> MPSQN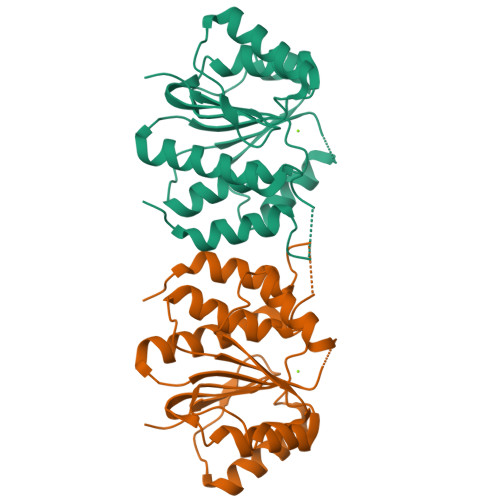ALYLDLLKKVLTNTIYSDRPHPNAWQDNTDYRQAARAKGTDWPTVAHTMIGLERLDNLQHCVEAVLADGVPGDFAETGVWRGGACIFMRAVLQAFGDTGRTVWVVDSFQGMPESSAQDHQADQAMALHEYNDVLGVSLETVRQNFARYGLLDEQVRFLPGWFRDTLPTAPIQELAVLRLDGDLYESTMDSLRNLYPKLSPGGFVIIDDYFLPSCQDAVKGFRAELGITEPIHDIDGTGAYWRRSWLEHHHHHH>GGGCUAAAAGCAUGGUGGGAAAGUGACGUGUAAUUCGUCCACAUUACUUGA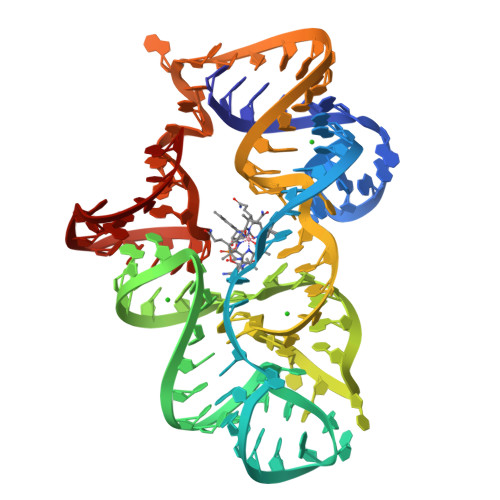UACGGUUAUACUCCGAAUGCCACCUAGCCCAAAGUAGAGCAAGGAGACUCA[2x]> GSHMQINLLNDFIKAYENTYSVSFDDSFKGRIQELCKELNEPFMHASYALENELKELVFSLDKN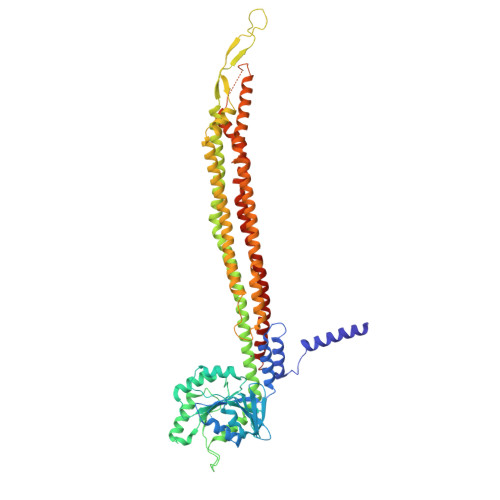VNIAIIGQFSSGKSSLLNLILGRDCLPTGVVPVTFKPTFLRYAKEYFLRVEFEDGSDIITNIEKLAFYTDQRNEVKQAKSLHIFAPIPLLEKITLVDTPGLNANENDTLTTLDELKNIHGAIWLSLIDNAGKKSEEDAIKANLELLGENSICVLNQKDKLSAEELDNVLNYAKSVFLKYFNELIAISCKEAKDEQSYEKSNFQSLLDFLTQLDTTVLKEKFVKRKILNLCEILEDENQLFVGIFDRLLNQFQSYEKHLLLAYENFLKEIEILNHQILEQLKSISERISSEIFASVKEKDAYFYKESKGFLKKDLYTRYDYKAPYISSDDAFLAMFYNSDVMSKEFKKIKNELYKSFEEIKMKLKDFINILEREILLFKAEFSNIQKDHIFQSDKNFSELRAFCNASDEYFLKDFKELLFKSILELDLFFEKLNLKAFTNYENATKLSLAFFSRKINESRVLYELDSSEFVLFYPKKSEIYERVLNELNVYEFETLLINKPILTKIAKNFLEQSQNLIQEKNKFLDLKKAELQKRRAQILNVRESIKEDHH Hedgehog-Interacting Protein (HHIP), the only reported secreted inhibitor of Sonic Hedgehog (SHH) signalling, binds directly to SHH with high nanomolar affinity, sequestering SHH. HHIP is composed of an N-terminal domain (HHIP-N) that shows weak sequence homology to the cysteine-rich domain (CRD) superfamily, typically involved in small molecule-binding. The C-terminal domain of HHIP is composed of a β-propeller and two EGF repeats (HHIP-C). Our data suggest a multimodal mechanism, in which HHIP can bind two specific sites on the SHH morphogen, alongside multiple GAG interactions, to inhibit SHH signalling.

We also determined the crystal structure of a HHIP-C:SOS complex, which exhibits the equivalent anti-parallel, dimeric HHIP arrangement bound to two SOS molecules coordinated at the same site compared to heparin. In summary, our HHIP-C crystal structures in complex with GAG molecules identify two discrete GAG-binding sites on the surface of HHIP-C, which are distinct and non-overlapping with the HhN-binding interface, thus suggesting that both GAG- and HhN-binding can occur simultaneously. To experimentally validate our HHIP-C:GAG complex structures, we generated a HHIP mutant in which 6 positively-charged residues involved in GAG recognition were mutated to glutamate (K277E/R328E/R350E/K569E/R610E/R613E, HHIP-C Glu mutant) and analysed binding to GAGs. Using surface plasmon resonance (SPR) with GAGs immobilised on the chip, we observed that the HHIP-C Glu mutant almost completely abolishes binding to heparin, HS and CS, when compared to wild-type (HHIP-C WT).

>[2x]ETGKHNCFCIQEVVSGLRQPVGALHSGDGSQRLFILEKEGYVKILTPEGEIFKEPYLDIHKLVQSGIKGGDERGLLSLAFHPNYKKNGKLYVSYTTNQERWAIGPHDHILRVVEYTVSRKNPHQVDLRTARVFLEVAELHRKHLGGQLLFGPDGFLYIILGDGMITLDDMEEMDGLSDFTGSVLRLDVDTDMCNVPYSIPRSNPHFNSTNQPPEVFAHGLHDPGRCAVDRHPTDININLTILCSDSNGKNRSSARILQIIKGKDYESEPSLLEFKPFSNGPLVGGFVYRGCQSERLYGSYVFGDRNGNFLTLQQSPVTKQWQEKPLCLGTSGSCRGYFSGHILGFGEDELGEVYILSSSKSMTQTHNGKLYKIVDPKRPLMPEECRATVQPAQTLTSECSRLCRNGYCTPTGKCCCSPGWEGDFCRTAKCEPACRHGGVCVRPNKCLCKKGYLGPQCEQVDGTKHHHHHH> SYYIDADLLREIKQHLKQQQEGLSHLI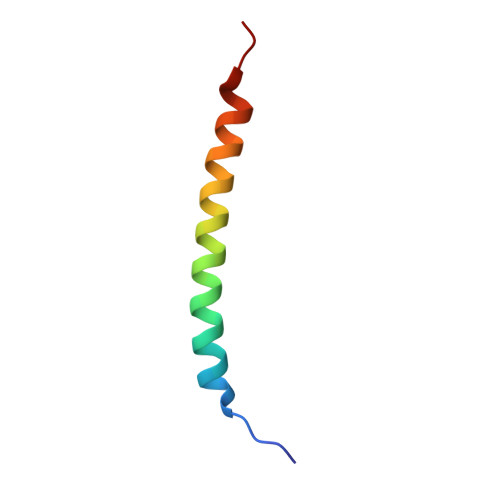SIIKDDLEDIKLV> MSTFEDADTEETVTCLQMTIYHPGQQSGIFKSIRFCSKEKFPSIEVVKFGRNSNMCQYTFQDKQVSRIQFVLQPFKQFNSSVLSFEIKNMSKKTSLMVDNQELGYLNKMDLPYKCMLRFGEYQFLLQKEDGESVESFETQFIMSSRPLLQENNWPTQNPIPEDGMYSSYFTHRSSPSEMDENELLEHHHHHH

TRAF-interacting protein with a forkhead-associated (FHA) domain (TIFA) was originally identified as an adaptor protein that interacts with TRAF2 and TRAF61–3. TIFA has an FHA domain, involved in its binding to phosphothreonine (pThr), and has a consensus TRAF6-binding motif [PXEXX(Ar/Ac); Ar, aromatic; Ac, acidic; X, any] at the C-terminus for interaction with the TRAF-C domain of TRAF6 (TRAF6-C). Furthermore, oligomeric forms of TIFA promote oligomerisation and polyubiquitination of TRAF6, leading to the activation of IκB kinase (IKK). TIFA exists as an intrinsic dimer, and phosphorylation of TIFA at Thr9 promotes its oligomerisation through the intermolecular interaction of pThr9 with the FHA domain between the dimers.

Full-length mouse TIFA with a C-terminal His tag was crystallised not only to reveal the structure of mouse TIFA, but also to elucidate its molecular assembly in a crystal. Mouse TIFA is composed of twelve β-strands (β-1 to β-12) and adapts a β-sandwich structure. Electron densities of nine N-terminal residues (Met1 to Thr9) including the phosphorylation site, and 43 C-terminal residues including the TRAF6-binding motif (from Gln150 to Leu184 and His tag) are missing, which indicates flexibility of the N- and C-terminal regions in the crystal. The overall structure is very similar to that of human TIFA, except for the region between β-1 and β-2 (from Ser27 to Ser37 in mouse TIFA) with root mean square deviation (r.m.s.d.) of 0.7 Å for the corresponding 128 Cα atoms. In the region between β-1 and β-2, structural diversity between mouse and human TIFA is observed due to either a deletion or an insertion in the amino acid sequence. The overall structure of the dimer is very similar to that of human TIFA, with r.m.s.d. of 0.9 Å for the corresponding 256 Cα atoms. The dimer of mouse TIFA, related by a crystallographic two-fold symmetry, is formed by van der Waals contacts and hydrogen bonding interactions at β-5, β-6, and β-9. In the centre of the dimer interface, a hydrogen bonding network is formed between Lys108, Glu86, and Asp110. In addition, there are hydrogen bonds between Gln73 residues, between Ser43 and Tyr105, between Lys88 and Pro74 (main chain), and between Asn107 and Lys76 (main chain). In total, fourteen hydrogen bonds appear to contribute to the dimer formation.2-[(4-methylsulfonyl-2-nitro-phenyl)-oxidanyl-methylidene]cyclohexane-1,3-dione | C14 H13 N 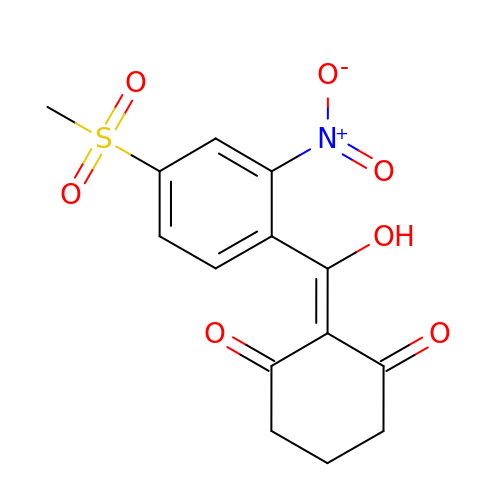O7 S | PILIZHLSOWYJPQ-UHFFFAOYSA-N Class X myosin has been found to be localized at the tips of filopodia, which are plasma membrane protrusions containing bundled actin that are necessary for cellular processes such as cell adhesion, migration, angiogenesis and the formation of cell–cell contacts. Myosin X is required for filopodia formation and extension. Myosin motors move along actin filaments via a series of conformational changes in the motor domain that are coupled with the sequential release of MgATP hydrolysis products, Pi and MgADP. These conformational changes in the motor domain are amplified by the myosin lever arm, which is comprized of the C-terminal subdomain of the motor domain (known as the converter) and an extended alpha helix length that varies with the myosin class12.

To compare the structure of this pre-powerstroke state with that of class V myosins, we attempted to crystallized myosin Va in this state but were unsuccessful. However, a data set was obtained from crystals of the motor domain of myosin Vc with two molecules in the asymmetric unit. These two myosin Vc molecules have quite similar structures for their motor domain but differ in the orientation of the converter. In contrast to myosin X, lack of interaction allows the myosin Vc converter to explore slightly different orientations. Comparison of these PPS structures show that while the subdomains of the motor are totally conserved in position among the myosin PPS structures obtained to date, the myosin X converter is rotated compared with that of myosin Vc and other myosins.

>[2x]ELYTQYNRVWIPDPEEVWKSAEIAKDYRVGDKVLRLLLEDGTELDYSVNPESLPPLRNPDILVGENDLTALSYLHEPAVLHNLRIRFAESKLIYTYSGIILVAMNPYKQLPIYGDAIIHAYSGQNMGDMDPHIFAVAEEAYKQMARNNRNQSIIVSGESGAGKTVSARYAMRYFATVSKSGSNAHVEDKVLASNPITEAVGNAKTTRNDNSSRFGKYTEISFDEQNQIIGANMSTYLLEKSRVVFQSENERNYHIFYQLCASAQQSEFKHLKLGSAEEFNYTRMGGNTVIEGVNDRAEMVETQKTFTLLGFKEDFQMDVFKILAAILHLGNVQITAVGNERSSVSEDDSHLKVFCELLGLESGRVAQWLCNRKIVTSSETVVKPMTRPQAVNARDALAKKIYAHLFDFIVERINQALQFSGKQHTFIGVLDIYGFETFDVNSFEQFCINYANEKLQQQFNMHVFKLEQEEYMKEDIPWTLIDFYDNQPVIDLIEAKMGILELLDEECLLPHGTDENWLQKLYNNFVNRNPLFEKPRMSNTSFVIQHFADKVEYKCEGFLEKNRDTVYDMLVEILRASKFHLCANFFQENPTPPSPFGSMITVKSAKQVIKPNSKHFRTTVGSKFRSSLYLLMETLNATTPHYVRCIKPNDEKLPFEFDSKRIVQQLRACGVLETIRISAQSYPSRWTYIEFYSRYGILMTKQELSFSDKKEVCKVVLHRLIQDSNQYQFGKTKIFFRAGQVAYLEKLRLD4-[3-(1H-benzimidazol-2-yl)-1H-indazol-6-yl]-3-ethylphenol | C22 H18 N4 O | 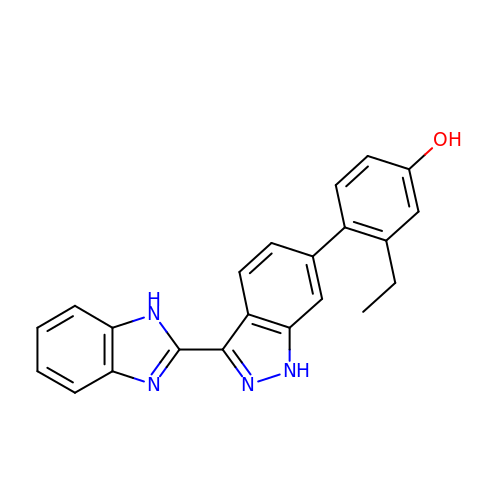CSLGOZXFBHTYAA-UHFFFAOYSA-N> MDPLCAAPCSCDGDRRVDCSGKGLTAVPEGLSAFTQALDISMNNITQLPEGAFKNFPFLEELQLAGNDLSFIHPKALSGLKELKVLTLQNNQLKTVPSEAIRGLSALQSLRLDANHITSVPEDSFEGLVQLRHLWLDDNSLTEV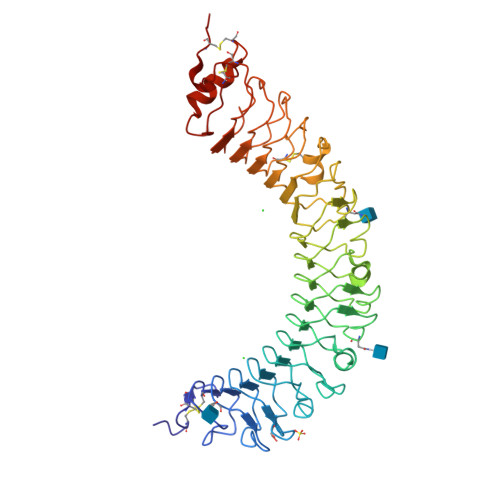PVHPLSNLPTLQALTLALNKISSIPDFAFTNLSSLVVLHLHNNKIRSLSQHCFDGLDNLETLDLNYNNLGEFPQAIKALPSLKELGFHSNSISVIPDGAFDGNPLLRTIHLYDNPLSFVGNSAFHNLSDLHSLVIRGASMVQQFPNLTGTVHLESLTLTGTKISSIPNNLCQEQKMLRTLDLSYNNIRDLPSFNGCHALEEISLQRNQIYQIKEGTFQGLISLRILDLASNQLKSVPDGIFDRLTSLQKIWLHTNPWDCSCPRIDYLSRWLNKNSQKEQGSAKCSGSGKPVRSIICPTL> MTTQQLKEKISKIIDNFSGIRVVFTTTANELKLSRIEGSALNSIAEGFIDKIKEDIINNEDLTSPLLSNFDDRKNALFKFDYEQYPEEFNKITQAIAIPPNSQDYYNPLNKFTDVKGIIILISGDNKCLALYKNKTNLAVLRNSRKMFNLVPDPDGYLKQLPNEILRLDFNYDLFSIGEDFYIKNHKTLETQMKFHQVIEAQAVI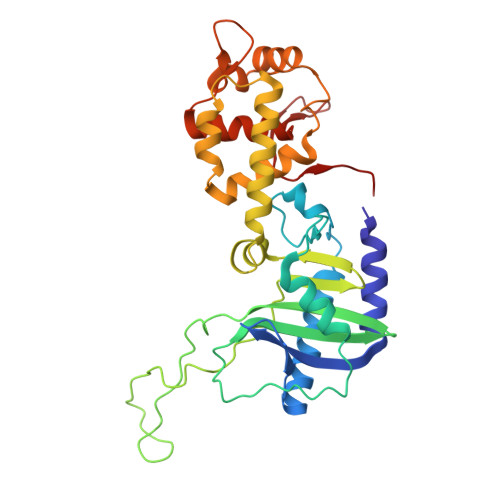ALNSLRDSLLIEDISGLEKSSREISFARKLAKISKHSPVLGKIDTKTIIDYVSQHKYLSAILQINEAGDKLLIKTKTSQKHFIKLMSDDYLQSDLTKIIYMSIAKDRLDE>[6x]GALERLPDGPRIHVPRKTALRPTVARQVFQPAFAPAVLSKFDPRTDADVDEVAFSKHTSNQETLPPVFRMVAREYANRVFALLGRDNGRLSVKQALDGLEGMDPMDKNTSPGLPYTTLGMRRTDVVDWETATLIPFAAERLEKMNNKDFSDIVYQTFLKDELRPIEKVQAAKTRIVDVPPFEHCILGRQLLGKFASKFQTQPGLELG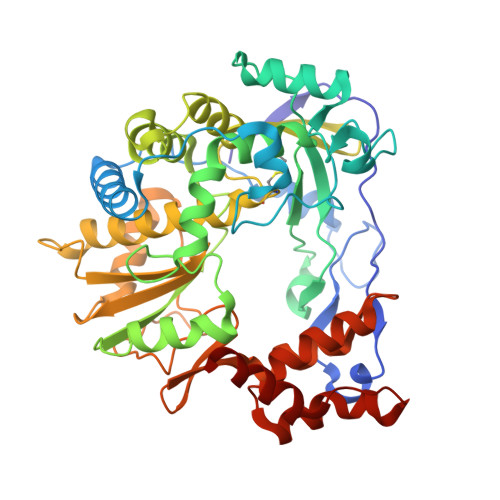SAIGCDPDVHWTAFGVAMQGFERVYDVDYSNFDSTHSVAMFRLLAEEFFSEENGFDPLVKDYLESLAISKHAYEEKRYLITGGLPSGCAATSMLNTVMNNIIIRAGLYLTYKNFEFDDVKVLSYGDDLLVATNYQLNFDRVRTSLAKTGYKITPANKTSTFPLESTLEDVVFLKRKFKKEGPLYRPVMNREALEAMLSYYRPGTLSEKLTSITMLAVHSGKQEYDRLFAPFREVGVIVPTFESVEYRWRSLFW> HHHHHHSSGLVPRGSHMRNYCTKTFGSAFSVTVVPTLKDNFSYLINDHTTHTLAAVDVNADYKPILTYIEEHLKQQGNADVTYTFSTILSTHKHWDHSGGNAKLKAELEAMNSTVPVVVVGGANDSIPAVTKPVREGDRVQVGDLSVEVIDAPCHTRGHVLYKVQHPQHPNDGVALFTGDTMFIAGIGAFFEGDEKDMCRAMEKVYH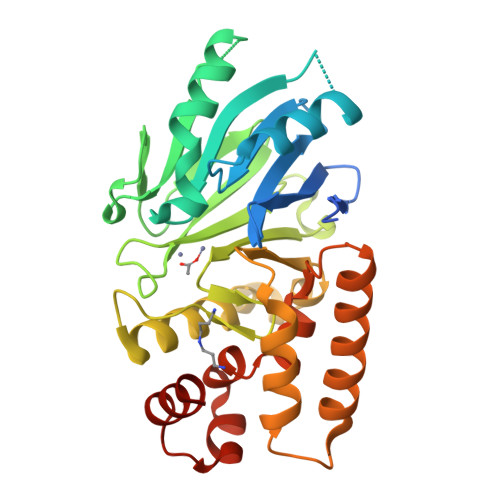IHKGNDYALDKVTFIFPGHEYTSGFMTFSEKTFPDRASDDLAFIQAQRAKYAAAVKTGDPSVPSSLAEEKRQNLFLRVADPAFVAKMNQGNAHALMMYLYNACD> 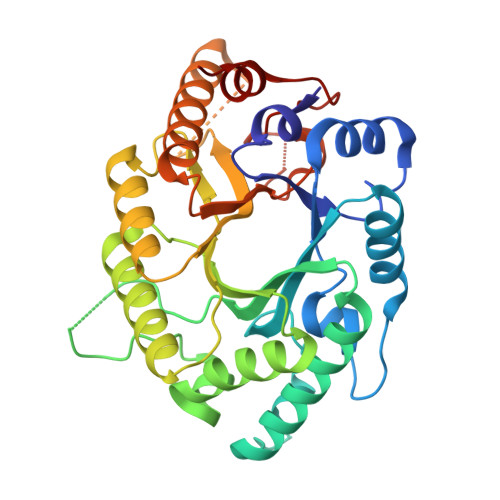NNLKDAYADYFTIGCAVNMANFNSSQQIALITSNFNSITAENDMKPQPTQPAEGKWNWENADKIANFARAHKIGLRGHCLVWHAQTGDWMFHDEKGDLVSKEVLFERMRTHIHTIVNRYKDVVYAWDVVNEAMTDDAKAEIPYRQSLYYKIAGDEFIKKAFEYAHEADPKALLFYNDYNETNPAKRDRIYNMVKSMKAEGIPISGIGMQGHYNVLSPTEDEFRKALELYSQVVDNIHITELDVRINTREQGGQLSVNQEGKKLELTPEADAAQVAQYDMLFRVMRDYKHVISNVTFWNGYDGDSWLDRRWGNRQRNYPLLFDENLLPKSSFSSYYKVL> XRMKQIEDKIEEIESKQKKIENE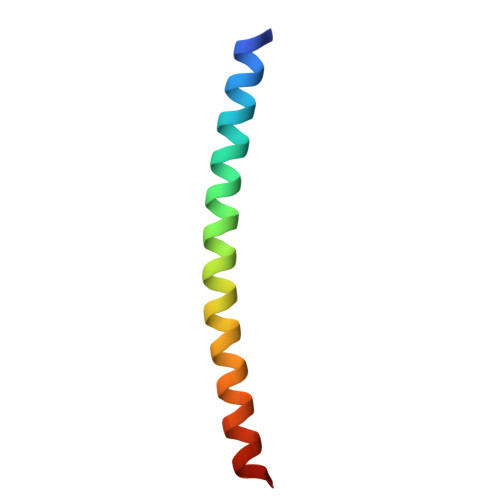IARIKKLLQLTVWGIKQLQARILX>[6x]MGSSHHHHHHSQDPSDQYPQTGTYP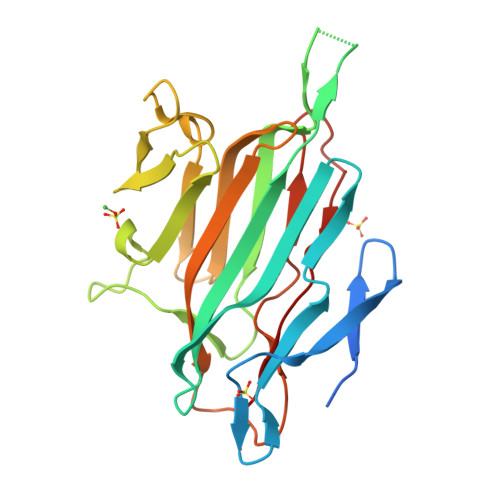DVQTPYQIIKVDGSEKNGQHKALNPNPYERVIPEGTLSKRIYQVNNLDDNQYGIELTVSGKTVYEQKDMADLTEKKSIENGTITDPMGELIDLQLGTDGRFDPADYTLTANDGSRLENGQAVGGPQNDGGLLKNAKVLYDTTEKRIRVTGLYLGTDEKVTLTYNVRLNDEFVSNKFYDTNGRTTLHPKEVEQNTVRDFPIPKIRDVR>[2x]MAHHHHHHVDDDDKMVTAAKGRIIGYVPGWKTPPAAQELASAGYTHVMIAFGVFSTNTPGVIVPAFETITKEYIQSLHQAGIKVILSLGGALTSIPNTTVDFHQVLVASSSPEAFKQTFINSLKELISQYGFDGFDTDIEHGINASGSFSQPQGDIAVLASIINTMYSQNSSLLITLTPQVANIAATSGFDQTWGNYASLIMQTHQSLAWVGIQLYNTGCAFGIDQVCYGPTPTDTPDFSVAMATDLLENWPATVNGRPTGFQPYISYLRPSQIVIGYPSPNASGGSDGSPVTPTTTIKRAIQCLKTAIAGNTSCGVYVPPRAYGNIGGVFNWEVTYDKNNQFKFAKELKNCAINGVCE

Among the L. pneumophila type II substrates, ChiA is an 81 kDa endochitinase with a novel amino acid sequence at its N-terminus and a putative glycosyl hydrolase 18 (GH18) domain at its C-terminus. ChiA is composed of four domains (N1, N2, N3 and CTD, from N- to C-terminus) which have structural homology to those associated with other chitinase enzymes. Using chitin binding and chitinase activity assays, we show that ChiA-N1 is a chitin binding module and we confirm that ChiA-CTD is a glycosyl hydrolase domain. Lastly, our structural and biochemical studies demonstrate that ChiA-CTD has novel peptidase activity against mucin-like glycoproteins, which is independent of its chitinase active site.

We readily obtained crystals for ChiA-CTD and its structure was determined using iodide single isomorphous replacement with anomalous scattering (I-SIRAS) phasing. Electron-density maps were refined to 1.7 Å and the final model contains two identical chains, with all molecules built except for the N-terminal His6-tags and adjacent ChiA-CTD residues Val419 to Gly424. Each chain forms an anticipated GH18 α/β-fold and is composed of 11 β-strands and 13 α-helices. High concentrations of 2-methyl-2,4-pentanediol (MPD) were used as a precipitant during crystallization and we observed four MPD molecules in the final model; one bound to the catalytic Asp541 and Glu543 residues (MPD-1) and one within a hydrophobic pocket formed by the α5 helix and α5-α5′/β5-β6′ loops (MPD-2). The chitinase active sites of ChiNCTU2 and ChiA-CTD have high primary sequence identity and tertiary structure homology and modelling of chitotetraose binding indicates that chitin lines a negatively charged valley on the surface of ChiA-CTD. Chitotetraose overlays with MPD-1 in the active site and the MPD-2 site is positioned adjacent to the reducing end of the modelled chitotetraose. However, L. pneumophila ChiA-CTD also possesses unique features that are not observed in homologous structures. These include an additional α-helix (α3), an extended β3-α3 loop, an extended α6-α6′ loop and an extended β7-α7 loop. Examination of the ChiA-CTD structure suggests that His544, Asn547 and Gln595 are ligands for the zinc, with Asp504 the general base. Furthermore, the MPD-2 site which we observed in the crystal structure of ChiA-CTD may also represent an additional glycan surface to accommodate branched glycan structures.>MRGSHHHHHHGSENLYFQSGAMEIREQLNLGGIVNAQNAQLSNCSDGAAQLESCGTAPDLKGITGWLNTPGNKPIDLKSLRGKVVLIDFWAYSCINCQRAIPHVVGWYQAYKDSGLAVIGVHTPEYAFEKVPGNVAKGAANLGISYPIALDNNYATWTNYRNRYWPAEYLIDATGTVRHIKFGEGDYNVTET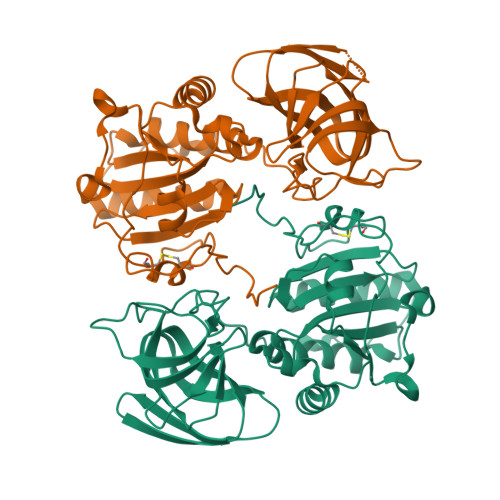LVRQLLNDAKPGVKLPQPSSTTTPDLTPRAALTPETYFGVGKVVNYGGGGAYDEGSAVFDYPPSLAANSFALRGRWALDYQGATSDGNDAAIKLNYHAKDVYIVVGGTGTLTVVRDGKPATLPISGPPTTHQVVAGYRLASETLEVRPSKGLQVFSFTYG[4x]>[4x]MEGISIYTSDNYTEEMGSGDYDSMKEPCFREENANFNKIFLPTIYSIIFLTGIVGNGLVILVMGYQKKLRSMTDKYRLHLSVADLLFVITLPFWAVDAVANWYFGNFLCKAVHVIYTVNLYSSVLILAFISLDRYLAIVHATNSQRPRKLLAEKVVYVGVWIPALLLT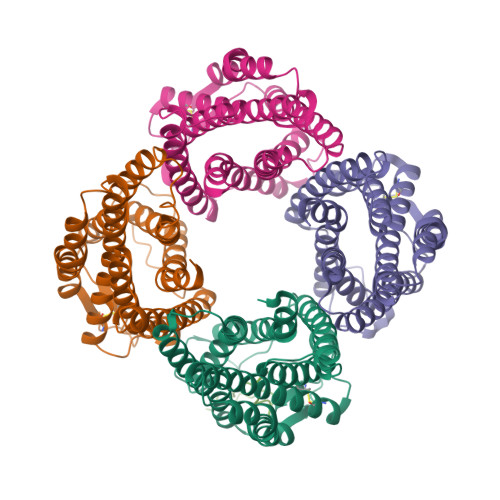IPDFIFANVSEADDRYICDRFYPNDLWVVVFQFQHIMVGLILPGIVILSCYCIIISKLSHSKGHQKRKALKTTVILILAFFACWLPYYIGISIDSFILLEIIKQGCEFENTVHKWISITEALAFFHCCLNPILYAFLGAKFKTSAQHALTSVSRGSSLKILSKGKRGGHSSVSTESESSSFHSSDYKDDDDK;> NKTVLPIMSGFKFHSKPVIN> MENKTETTVRRRRRIILFPVPFQGHINPILQLANVLYSKGFSITIFHTNFNKPKTSNYPHFTFRFILDNDPQDERISNLPTHGPLAGMRIPIINEHGADELRRELELLMLASEEDEEVSCLITDALWYFAQSVADSLNLRRLVLMTSSLFNFHAHVSLPQFDELGYLDPDDKTRLEEQASGFPMLKVKDIKSAYSNWQILKEILGKMIKQ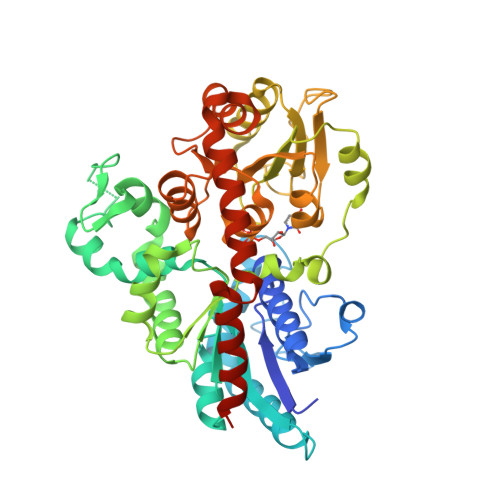TKASSGVIWNSFKELEESELETVIREIPAPSFLIPLPKHLTASSSSLLDHDRTVFQWLDQQPPSSVLYVSFGSTSEVDEKDFLEIARGLVDSKQSFLWVVRPGFVKGSTWVEPLPDGFLGERGRIVKWVPQQEVLAHGAIGAFWTHSGWNSTLESVCEGVPMIFSDFGLDQPLNARYMSDVLKVGVYLENGWERGEIANAIRRVMVDEEGEYIRQNARVLKQKADVSLMKGGSSYESLESLVSYISSLLEHHHHHH>GSQSGPLPKPSLQALPSSLVPLEKPVTLRCQGPPGVDLYRLEKLSSSRYQDQAVLFIPAMKRSLAGRYRCSYQNGSLWSLPSDQLELVATGVFAKPSLSAQPGSGGDVTLQCQTRYGFDQFALYKEGDPERWYRASFPIITVTAAHSGTYRCYSFSSRDPYLWSAPSDPLELVVTGTSAAA[2x];>[3x]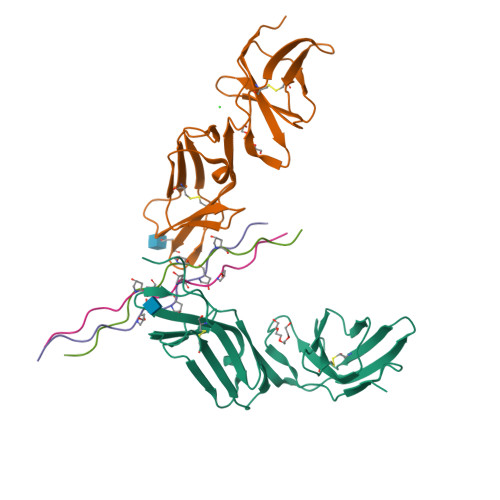GPPGPPGPPGPPGPPGPPGPP> METAIWIKNSKLPAVLVAAGAFDAAVQALSKQVGVVKLEPLKKYFTNIYEGCRTYIPSTPCELPAQLGYVRAYDDTVSEDQILPYVPGLDVVNEKMNEGYKNFKLNKPDIAIECFREAIYRITLLMVDDAEDEKLAHKILETAREYILGLSIELERRSLKEGNTVRMLELAAYFTKAKL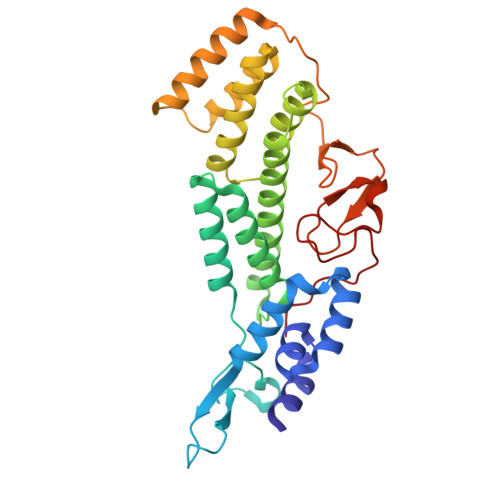SPIHRTNALQVAMSQHFKHKNFLQASYFAGEFLKIISSGPRAEQARKIKNKADSMASDAIPIDFDPYAKFDICAATYKPIYEDTPSVSDPLTGSKYVITEKDKIDRIAMISKIGAPASGLRIRV> MLAKDKVALLIGNMNYREHPKLKAPLVDVY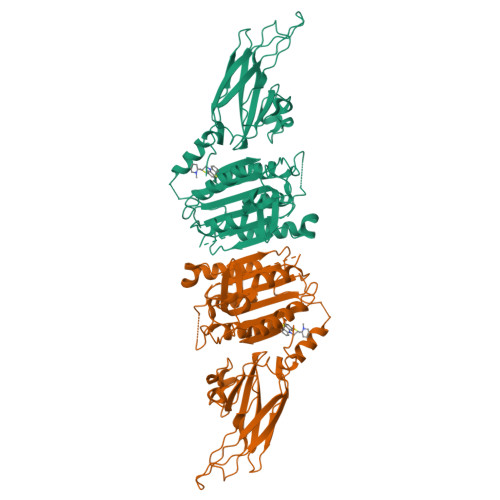ELTNLLRQLDFKVVSLLDLTEYEMRNAVDEFLLLLDKGVYGLLYYAGHGYENFGNSFMVPVDAPNPYRSENCLCVQNILKLMQEKETGLNVFLLDMCRKRNDYDDTIPILDALKVTANIVFGYATCQGAEAFEIQHSGLANGIFMKFLKDRLLEDKKITVLLDEVAEDMGKCHLTKGKQALEIRSSLSEKRALTDPIQGTEYSAESLVRNLQWAKAHELPESMCLKFDCGVQIQLGFAAEFSNVMIIYTSIVYKPPEIIMCDAYVTDFPLDLDIDPKDANKGTPEETGSYLVSKDLPKHCLYTRLSSLQKLKEHLVFTVCLSYQYSGLEDTVEDKQEVNVGKPLIAKLDMHRHHHHHH>MALQRTLSIIKPDAVSKNVIGEILTRFEKAGLRVVAAKMVQLSEREAGGFYAEHKERPFFKDLVSFMTSGPVVVQVLEGEDAIAKNRELMGATDPKKADAGTIRADFAVSIDENAVHGSDSEASAAREIAYFFAAT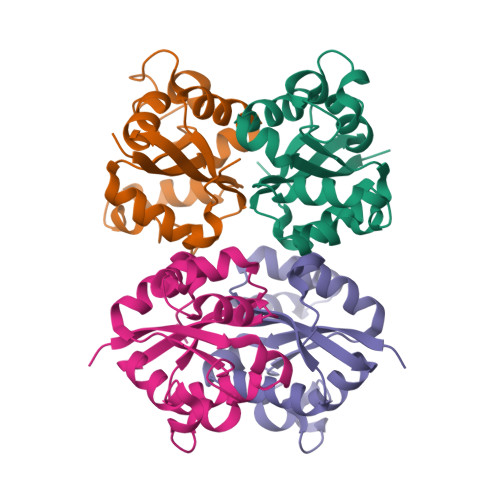EVCERIR[8x]>[2x]ATFLIWPIY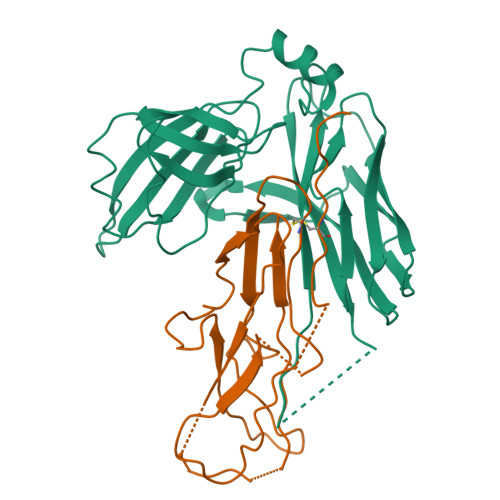PKIEANEKATAVWLQNTGKTDAMVQIRVFKWNQDGLKDNYSEQSEIIPSPPVAKIKAGEKHMLRLTKSVNLPDGKEQSYRLIVDELPIRLSDGNEQDASKVSFQMRYSIPLFAYGKGIGSGLTEESQKLNAKNALAKPVLQWSVRNNQQGQSELYLKNNGQKFARLSALKTSKTGNDISLGKAAFGYVLSNSTVKFAIDQSTAHELAKTSKIYGVDSSGIKQELIEITKMEDPS;>[2x]AVTHHHHHHSTGCTVGGSQTEGNMNKFGTLNFGKTSGTWNNVLTAEVASAATGGNISVTCDGTDPVDFTVAIDGGERTDRTLKNTASADVVAYNVYRDAARTNLYVVNQPQQFTTVSGQATAVPIFGAIAPNTGTPKAQGDYKDTLLVTVNF> MTSRKKVLLKVIILGDSGVGKTSLMNQYVNKKFSNQYKATIGADFLTKEVMVDDRLVTMQIWDTAGLERFQSLGVAFYRGADCCVLVFDVTAPNTFKTLD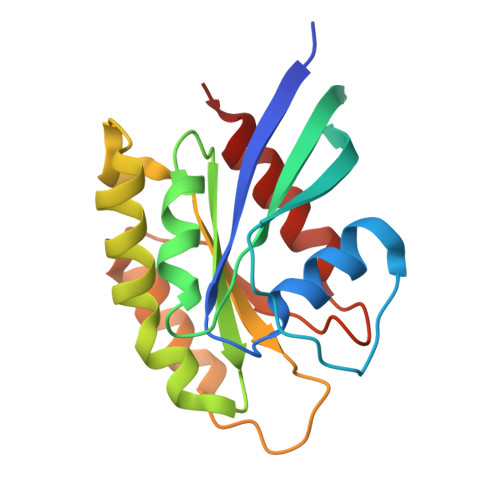SWRDEFLIQASPRDPENFPFVVLGNKIDLENRQVATKRAQAWCYSKNNIPYFETSAKEAINVEQAFQTIARNALKQ>MVLYFIGLGLYDERDITVKGLEIAKKCDYVFAEFYTS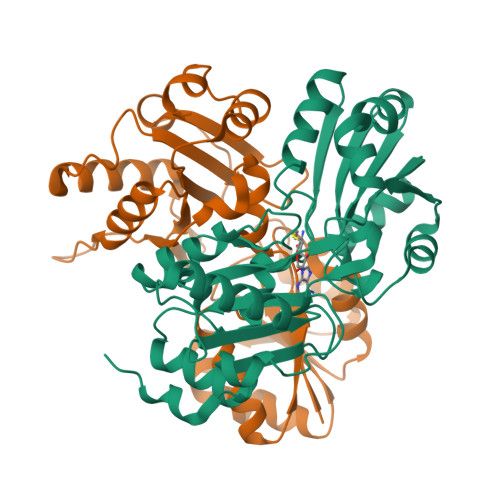LMAGTTLGRIQKLIGKEIRVLSREDVELNFENIVLPLAKENDVAFLTPGDPLVATTHAELRIRAKRAGVESYVIHAPSIYSAVGITGLHMYKFGKSATVAYPEGNWFPTSYYDVIKENAERGLHTLLFLDIKAEKRMYMTANEAMELLLKVEDMKKGGVFTDDTLVVVLARAGSLNPTIRAGYVKDLIREDFGDPPHILIVPGKLHIVEAEYLVEIAGAPREILRVNV[2x]>MEDLNVVDSINGAGSWLVANQALLLSYAVNIDFICTSLIAVILTIKLFLLINQFEKQQIKKGRDITSARIM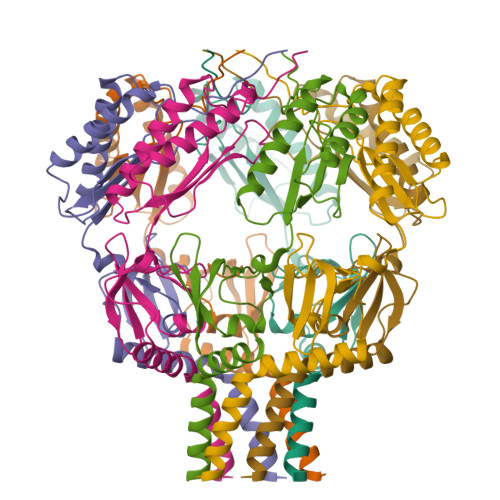SRIIKITIIVVLVLLYGEHFGMSLSGLLTFGGIGGLAVGMAGKDILSNFFSGIMLYFDRPFSIGDWIRSPDRNIEGTVAEIGWRITKITTFDNRPLYVPNSLFSSISVENPGRMTNRRITTTIGLRYEDAAKVGVIVEAVREMLKNHPAIDQRQTLLVYFNQFADSSLNIMVYCFTKTTVWAEWLAAQQDVYLKIIDIVQSHGADFAFPSQTLYMDNITPPEQGRAAALEHHHHHH[7x]>[6x]MEYKSTRHAKY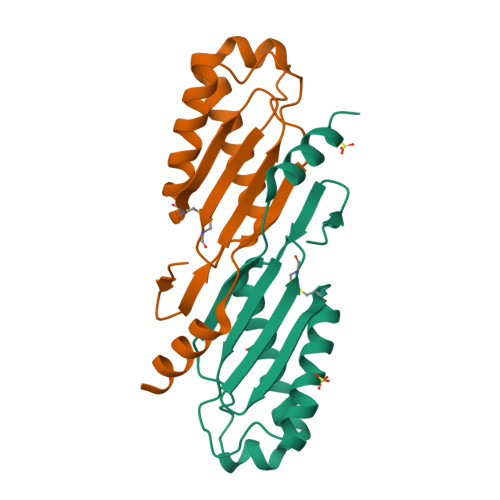LCNYHFVWIPKYRRKVLTGEVAEYTKEVLRTIAEELGCEVLALEVMPDHIHLFVNCPPRYAPSYLANYFKGKSARLILKKFQELKKSTNGKLWTRSYFVSTSGNVSSETIKKYIEEQWAKENEED Here, we report the discovery and characterization of a new FAD-dependent D-lactate dehydrogenase (PdG-D-LDH) from the gut microbiome of the isopod Porcellio dilatatus. PdG-D-LDH exhibits a strong catalytic preference toward D-lactate and preferentially reduces quinones over cytochrome c or molecular oxygen. X-ray crystallography revealed a VAO/PCMH-like fold with a solvent-accessible active site that harbors both a FAD cofactor and an Fe(II) ion. PdG-D-LDH exhibits the characteristic VAO/PCMH structural fold.

The crystal structure of the enzyme was solved both in the absence or presence of D-lactate (PdG-D-LDH–lactate), revealing a Cα root-mean-square deviation (RMSD) of 0.46 Å between the two structures. Moreover, a metal ion and the substrate D-lactate (in PdG-D-LDH-lactate complex) are clearly defined in the electron density. In D-LDH, D-lactate binds Fe(II) and interacts with H416, which likely abstracts a proton from the C2-OH, enabling hydride transfer to FAD’s N5. The C1 group coordinates iron and forms salt bridges with R323, while the C3 group engages in hydrophobic interactions with Y327, I369, and L380. In PdG-D-LDH, the C2-OH is 4.6 Å from FAD’s N5—too distant for efficient catalysis—unlike m-D-LDH, where this distance is 3.1 Å. Thus, the PdG-D-LDH–substrate complex likely lacks a catalytically competent geometry. The substrate-binding site comprises two distinct regions: one predominantly positively charged, defined by R323, H371, H378, and H416, is located near the C1-carboxyl and C2-hydroxyl groups of D-lactate. The other, more hydrophobic, is primarily delimited by Y327, I369, and L380, facilitating a stronger interaction with the substrate.

>[8x]MPGVVEELVAAIGAEQVVTDPAVMEGYSHDEAEWAPYDAPAAVVRPRDTADVAEVVRICAGRGVAVVGRGAGTGLSGAANAGRGWVVVSFERMNRVLEVDTVQQTVTVQPGVVNDDLRARVAQDGLWYPPDPASSPWSTIGGNVATNAGGLCCVKYGVTRDYVLGMEAVVGSGEVVRLGRTTAKGVTGYDLAGLMVGSEGTLGLVTEVTLRLVPLRRGVEHTVVGYFDSLTDAGRAVAAVSAAGIVPSALELIDRFCLQAVDEWKNMGLSAEGEVLLLARSDLPGTSGQEEADRILECFEKEKAVYAVRSTDEEEAEALFQARRLAYPALERLGPLLTEDVCVPKARVPHMLEAIEAAGERFDTRIGNIAHAGDGNLHPLFIVPAGDEEAKRRAKQAFEVIVDEALAVGGTVTGEHGVGLLKMRGAADELGPHVLAMHRAVKGALDPAGIFNPGKVFALEEERD>[2x]XLAAWLAQ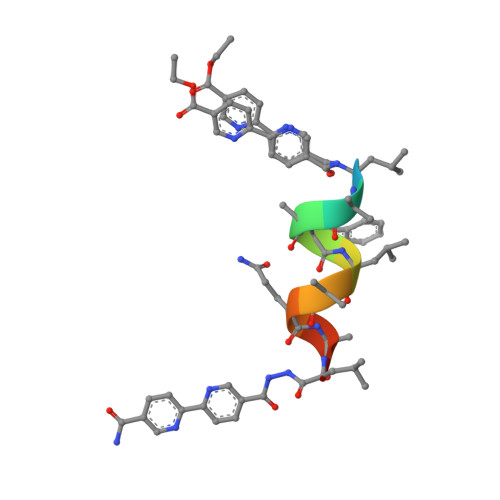ALX>[2x]GIKCFAVRSLGWVEMTEEELAPGRSSVAVNNCIRQLSYHKNNLHDPMSGGWGEGKDLLLQLEDE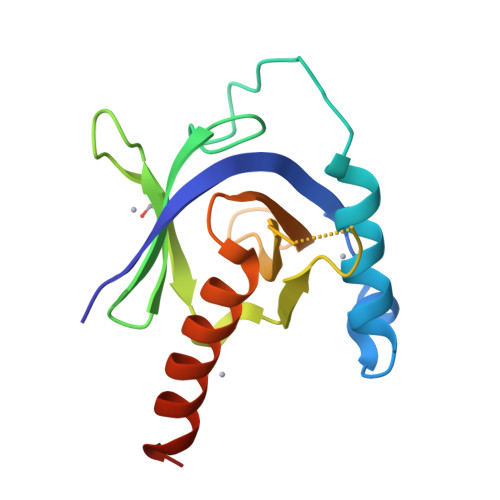TLKLVEPQSQALLHAQPIISIRVWGVGRDSGRERDFAYVARDKLTQMLKCHVFRCEAPAKNIATSLHEICSKIMAELEHHHHHH> 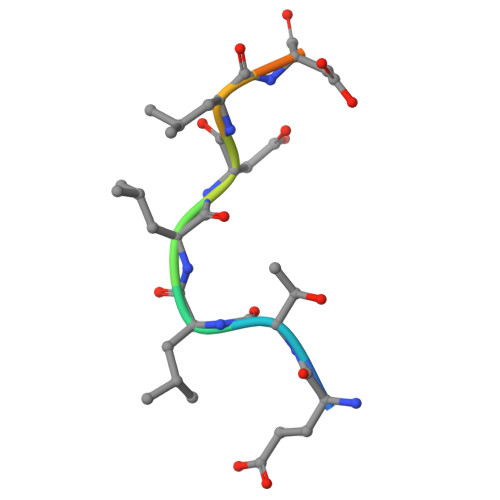ETLLDLDFLE> MNDIIINKIATIKRCIKRIQQVYGDGSQFKQDFTLQDSVILNLQRCCEACIDIANHINRQQQLGIPQSSRDSFTLLAQNNLITQPLSDNLKKMVGLRNIAVHDAQELNLDI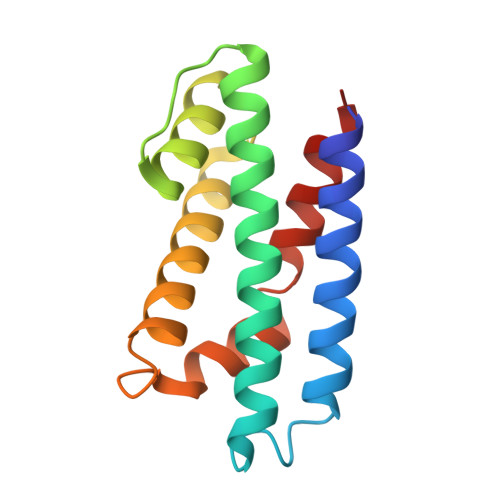VVHVVQHHLEDFEQFIDVIKAE>ASNTVMKNCNYKRKRRERDWDCNTKKDVCIPDRRYQLCMKELTNLVNNTDTNFHRDITFRKLYLKRKLIYDAAVEGDLLLKLNNYRYNKDFCKDIRWSLGDFGDIIMGTDMEGIGYSKVVENNLRSIFGTDEKAQQRRKQWWNESKAQIWTAMMYSVKKRLKGNFIWICKLNVAVNIEPQIYRWIREWGRDYVSELPTEVQKLKEKCDGKINYTDKKVCKVPPCQNACKSYDQWITRKKNQWDVLSNKFISVKNAEKVQTAGIVTPYDILKQELDEFNEVAFENEINKRDGAYIELCVCSVEEAKKNTQEVVTNVDN[2x];> GPTGNSSQLDFEDVWNSSYGVNDSFPDGDYGA

DBP is a member of the erythrocyte binding-like (EBL) family of proteins, which localize to micronemes and use Duffy binding-like (DBL) domains to bind specific RBC receptors with high affinity. DBL domains are located in “region II” of EBL proteins, and DBP region II (DBP-RII) is required for formation of a tight junction between Plasmodium and RBC membranes. Two crystal forms were observed, a heterotrimeric complex in which one DARC molecule binds the DBP-RII dimer, and a heterotetrameric complex containing two DARC molecules bound to the DBP-RII dimer.

In this structure, two DBP-RIIs (DBP1 and DBP2) bind a single DARC (DARC A) creating the heterotrimer with a total buried surface area of 2241.8 Å2. Additionally, in the heterotrimer, the second DARC binding site is preformed to accept another DARC. In the heterotrimer structure, a new DBP-RII homodimer interface is created by a translation of 7 residues covering 12 Å along helix 4, relative to the unbound structure. The DBP-RII homodimer interface is composed of DBP1 residues I265-R274 and DBP2 residues F261-Y278 in the heterotrimer, and DBP1 residues H262-R274 and DBP2 residues F261-Y278 in the heterotetramer. In the heterotrimer, residues H262-T266 make contacts at the secondary interface. In addition to the dimer interface, each DARC binding site, one in the heterotrimer and two in the heterotetramer, can be broken into two interfaces: a primary DARC binding interface with one DBP-RII monomer, and a secondary DARC binding interface created by the second DBP-RII monomer. The primary DARC binding interface in both structures consists of DBP-RII residues L270-K289 of helix 4 and Q356-K367 of helix 7. DARC is induced to form an amphipathic helix in the crystal structures upon binding and engages a positively charged groove at the DBP-RII dimer interface. The heterotrimer and heterotetramer could represent DBP-RII binding to a DARC heterodimer or homodimer, respectively. Specifically, the two bound forms of DBP-RII observed in the crystal structures suggest that an initial binding event followed by receptor-induced DBP dimerization leads to a DBP∶DARC heterotrimer that subsequently binds to a second DARC monomer to create the final heterotetrameric assembly.> MAHHHHHHHHHHGALEVLFQGPGDPTVFHKRYLKKIRDLGEGHFGKVSLYCYDPTNDGTGEMVAVKALKADAGPQHRSGWKQEIDILRTLYHEHIIKYKGCCEDAGAASLQLVMEYVPLGSLRDYLPRHSIGLAQLLLFAQQICEGMAYLHAQHYIHRDLAARNVLLDNDRLVKIGDFGLAKAVPEG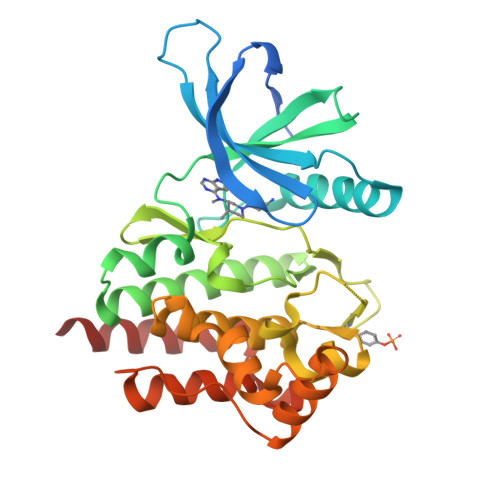HEYYRVREDGDSPVFWYAPECLKEYKFYYASDVWSFGVTLYELLTHCDSSQSPPTKFLELIGIAQGQMTVLRLTELLERGERLPRPDKCPAEVYHLMKNCWETEASFRPTFENLIPILKTVHEKYQGQAPS> MEVLFEAKVGDITLKLAQGDITQYPAKAIVNAANKRLEHGGGVAYAIAKACAGDAGLYTEISKKAMREQFGRDYIDHGEVVVTPAMNLEERGIKYVFHTVGPICSG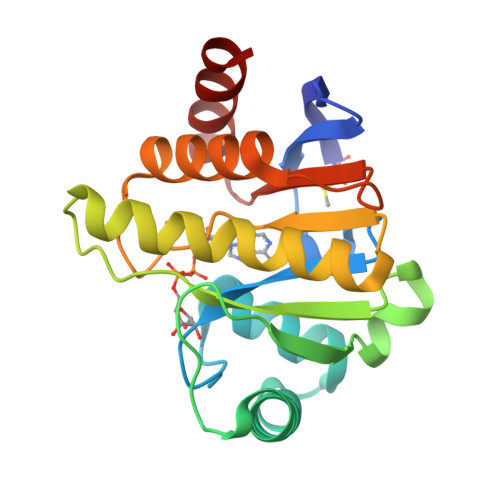MWSEELKEKLYKAFLGPLEKAEEMGVESIAFPAVSAGIYGCDLEKVVETFLEAVKNFKGSAVKEVALVIYDRKSAEVALKVFERSL> MVSAADVYVPDEWEVAREKITMSRELGQGSFGMVYEGVAKGVVKDEPETRVAIKTVNEAASMRERIEFLNEASVMKEFNCHHVVRLLGVVSQGQPTLVIMELMTRGDLKSYLRSLRPEMENNPVLAPPSLSKMIQMAGEIADGMAYLNANKFVHRDLAARNCMVAEDFTVKIGDFGMTRDIYETDYYRKGGKGLLPVRWMSPESLKDGVFTTYSDVWSFGVVLWEIATLAEQPYQGLSNEQVLRFVMEGGLLDKPDNCPDMLFELMRMCWQYNPKMRPSFLEIISS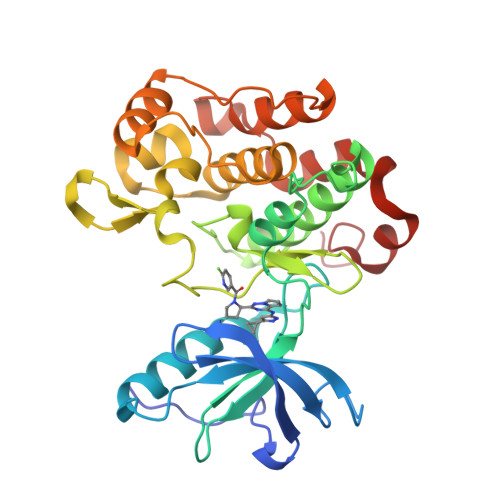IKEEMEPGFREVSFYYSEENK> MRERIREHLSSEESVGLLFSGCTGINDKTLGARGGEVIMVTSGSGMGKSTFVRQQALQWGTAMGKKVGLAMLEESVEETAEDLIGLHNRVRLRQSDSLKREIIENGKFDQWFDELFGNDTFHLYDSFAEAETDRLLAKLAYMRSGLGCDVIILDHISIVVS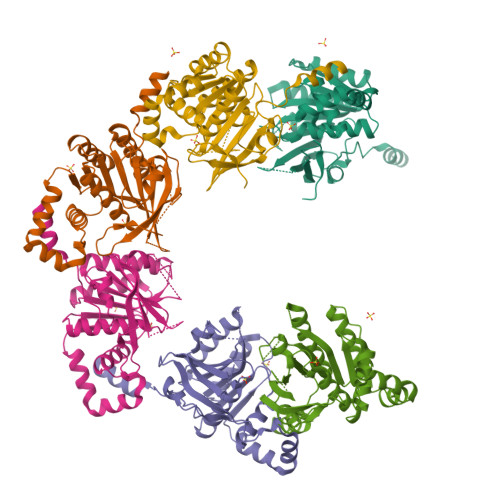ASGESDERKMIDNLMTKLKGFAKSTGVVLVVICHLKNPDKGKAHEEGRPVSITDLRGSGALRQLSDTIIALERNQQGDMPNLVLVRILKCRFTGDTGIAGYMEYNKETGWLEPSSYSGEEESHSESTDWSNDTDF>MFEARLVQGSILKKVLEALKDLINEACWDISSSGVNLQSMDSSHVSLVQLTLRSEGFDTYRCDRNLAMGVNLTSMSKILKCAGNEDIITLRAEDNADTLALVFEAPNQEKVSDYEMKLMDLDVEQLGIPEQEYSCVVKMPSGEFARICRDLSHIGDAVVISCAKDGVKFSASGELGNGNIKLSQTSNVDKEEEAVTIEMNEPVQLTFALRYLNFFTKATPLSSTVTLSMSADVPLVVEYKIADMGHLKYYLAPKIEDEEGS[3x];>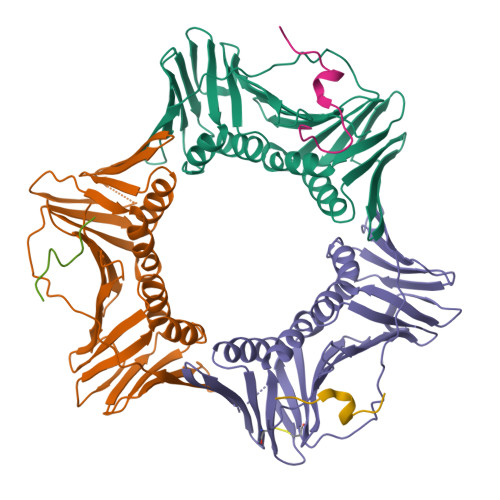CKRPRPEGMQTLESFFKPLTH[3x]During the early and late steps of infection with the Gram-positive bacterium B. anthracis, the tripartite anthrax toxin is secreted as major virulence factor in order to kill host immune cells such as macrophages or neutrophils. Like other AB-type toxins, it is composed of a surface binding/translocation moiety, the protective antigen (PA, 83 kDa), and two cytotoxic subunits, lethal factor (LF, 90 kDa) and edema factor (EF, 93 kDa). After cleavage by furin-like proteases, the truncated 63 kDa-sized PA monomer oligomerizes either into homo-heptamers (PA7) or homo-octamers (PA8). While PA8 can bind up to four factors, only three of them can simultaneously bind to PA7. Both enzymatic substrates bind to the upper rim of the PA oligomer via their N-terminal domains in a competitive manner.

We determined three structures of the fully-loaded heptameric anthrax lethal toxin complex, which differ in the position and conformations of the bound LFs. Due to a symmetry mismatch, three LFs occupy six binding sites of the heptameric PA7 complex, leaving one PA site empty. Binding of LF to a single PA protomer is mediated via the N-terminal domain of LF, orienting its bulky C-terminal domain such that the adjacent PA protomer is not accessible for binding. In this way a single lethal factor de facto occupies two of the seven binding sites of PA7. In the chain of LFs, the C-terminal domain of the anterior LF binds to the N-terminal domain of the following one, creating a directionality in the complex. Consequently, if two LFs are bound, three free PA binding sites are available, of which only two can potentially be occupied due to steric clashes. This results in the two complexes PA7LF2+1A and PA7LF2+1B, that differ in the binding position of the third LF. In two of our structures, PA7LF2+1A and PA7LF2+1B, two LFs only interact at one position which is located next to the major LF-PA interface. However, we only found that the N-terminal region of one LF (2LF) resides in the α-clamp, adopting the “open” conformation as described for PA8LF4. In the other LFs (1LF, 3LF), this region is flexible and not interacting with the α-clamp.

>MGHHHHHHHHHHSSGHIDDDDKHMEVKQENRLLNESESSSQGLLGYYFSDLNFQAPMVVTSSTTGDLSIPSSELENIPSENQYFQSAIWSGFIKVKKSDEYTFATSADNHVTMWVDDQEVINKASNSNKIRLEKGRLYQIKIQYQRENPTEKGLDFKLYWTDSQNKKEVISSDNLQLPELKQKSSNSRKKRSTSAGPTVPDRDNDGIPDSLEVEGYTVDVKNKRTFLSPWISNIHEKKGLTKYKSSPEKWSTASDPYSDFEKVTGRIDKNVSPEARHPLVAAYPIVHVDMENIILSKNEDQSTQNTDSQTRTISKNTSTSRTHTSEVHGNAEVHASFFDIGGSVSAGFSNSNSSTVAIDHSLSLAGERTWAETMGLNTADTARLNANIRYVNTGTAPIYNVLPTTSLVLGKNQTLATIKAKENQLSQILAPNNYYPSKNLAPIALNAQDDFSSTPITMNYNQFLELEKTKQLRLDTDQVYGNIATYNFENGRVRVDTGSNWSEVLPQIQETTARIIFNGKDLNLVERRIAAVNPSDPLETTKPDMTLKEALKIAFGFNEPNGNLQYQGKDITEFDFNFDQQTSQNIKNQLAELNATNIYTVLDKIKLNAKMNILIRDKRFHYDRNNIAVGADESVVKEAHREVINSSTEGLLLNIDKDIRKILSGYIVEIEDTEGLKEVINDRYDMLNISSLRQDGKTFIDFKKYNDKLPLYISNPNYKVNVYAVTKENTIINPSENGDTSTNGIKKILIFSKKGYEIG[7x];>[3x]MNIKKEFIKVISMSCLVTAITLSGPVFIPLVQGAGGHGDVGMHVKEKEKNKDENKRKDEERNKTQEEHLKEIMKHIVKIEVKGEEAVKKEAAEKLLEKVPSDVLEMYKAIGGKIYIVDGDITKHISLEALSEDKKKIKDIYGKDALLHEHYVYAKEGYEPVLVIQSSEDYVENTEKALNVYYEIGKILSRDILSKINQPYQKFLDVLNTIKNASDSDGQDLLFTNQLKEHPTDFSVEFLEQNSNEVQEVFAKAFAYYIEPQHRDVLQLYAPEAFNYMDKFNEQEINLSLEELKDQRMLARYEKWEKIKQHYQHWSDSLSEEGRGLLKKLQIPIEPKKDDIIHSLSQEEKELLKRIQIDSSDFLSTEEKEFLKKLQIDIRDSLSEEEKELLNRIQVDSSNPLSEKEKEFLKKLKLDIQPYDINQRLQDTGGLIDSPSINLDVRKQYKRDIQNIDALLHQSIGSTLYNKIYLYENMNINNLTATLGADLVDSTDNTKINRGIFNEFKKNFKYSISSNYMIVDINERPALDNERLKWRIQLSPDTRAGYLENGKLILQRNIGLEIKDVQIIKQSEKEYIRIDAKVVPKSKIDTKIQEAQLNINQEWNKALGLPKYTKLITFNVHNRYASNIVESAYLILNEWKNNIQSDLIKKVTNYLVDGNGRFVFTDITLPNIAEQYTHQDEIYEQVHSKGLYVPESRSILLHGPSKGVELRNDSEGFIHEFGHAVDDYAGYLLDKNQSDLVTNSKKFIDIFKEEGSNLTSYGRTNEAEFFAEAFRLMHSTDHAERLKVQKNAPKTFQFINDQIKFIINS BK polyomavirus is the causative agent of several diseases in transplant patients and the immunosuppressed. The crystal structures of these viruses revealed that polyomavirus capsids consist of 360 copies of the major capsid protein VP1 (Liddington et al., 1991). These VP1 molecules form 72 pentameric structures, or pentons, that form the basic building block (or capsomere) of the capsid. Each penton consists of a ring of five β-barrel-containing VP1 monomers (Nilsson et al., 2005). Together these form a T = 7d lattice, with an invading arm comprised of the C termini of each VP1 undergoing exchange with neighboring pentons to stabilize the capsid shell.

Images of unstained, frozen-hydrated virions and VLPs were recorded using an electron microscope with a direct electron-detecting camera, allowing us to determine the solution structures of the virion to 7.6 Å and VLP to 9.1 Å. Each penton contains five copies of the major structural protein VP1, and there are six distinct conformations of VP1 in the shell. A homology model of the BK VP1 asymmetric unit was generated based on SV40 using the SWISS-MODEL server and flexibly fitted into the corresponding density of the virion map. At the resolution presented, the gross fold of BK VP1 is extremely similar to previous structures of the non-human polyomavirus, SV40, which shares 81.7% sequence identity in the major structural protein. Strong density is observed inside the virion, as two ∼24-Å thick radial shells separated by a gap of ∼28 Å. Interestingly, the density associated with the N termini of chains 3 and 6 appear to be a weaker feature within the virion map. We propose that these densities correspond to some portion of the 13–15 N-terminal residues of VP1, which are not resolved in previous polyomavirus structures.

>[6x]MAPTKRKGECPGAAPKKPKEPVQVPKLLIKGGVEVLEVKTGVDAITEVECFLNPEMGDPDENLRGFSLKLSAENDFSSDSPERKMLPCYSTARIPLPNLNEDLTCGNLLMWEAVTVQTEVIGITSMLNLHAGSQKVHEHGGGKPIQGSNFHFFAVGGEPLEMQGVLMNYRSKYPDGTITPKNPTAQSQVMNTDHKAYLDKNNAYPVECWVPDPSRNENARYFGTFTGGENVPPVLHVTNTATTVLLDEQGVGPLCKADSLYVSAADICGLFTNSSGTQQWRGLARYFKIRLRKRSVKNPYPISFLLSDLINRRTQRVDGQPMYGMESQVEEVRVFDGTERLPGDPDMIRYIDKQGQLQTKML>MRLFSLSTALSSAMIALVSLPLQAAAPAQQKTQVPGYYRMALGDFEVTALYDGYVDLPASLLKGIDDKDLQSLLARMFVASEKGVQTAVNAYLINTGDNLVLIDTGAAQCFGPTLGVVQTNLKASGYQPEQVDTVLLTHLHPDHACGLVNADGSPAYPNATVEVPQAEAEFWLDEATMAKAPEGMQGMFKMARQAVAPYAKMNKLKPYKTEGELLPGVSLVASSGHTPGHTSYLFKSGGQSLLVWGDILINHAVQFAKPEVVWEFDVDSDQARQSRQRILAEAATDKLWVAGAHLPFPGLGHVREEAQGYAWVPVEFSPIRSD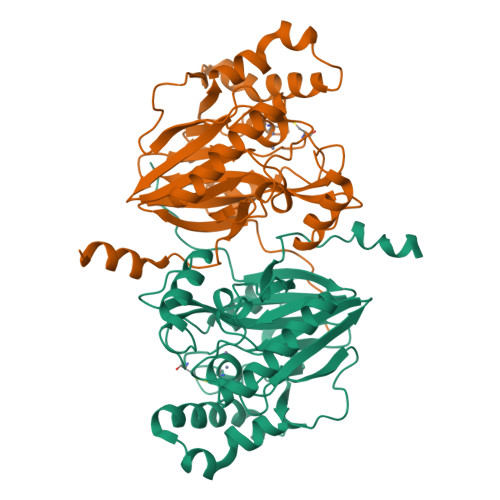RKLAAALEHHHHHH[2x]> MGRDPNSTNDTTTQNVVLTKYGFDKDVTAIDRATDQIWTGDGAKPLQGVDFTIYNVTANYWASPKDYKGSFDSAPVAATGTTNDKGQLTQALPIQSKDASGKTRAAVYLFHETNPRAGYNTSADFWLTLPAKAAADGNVYVYPKNVQKTTY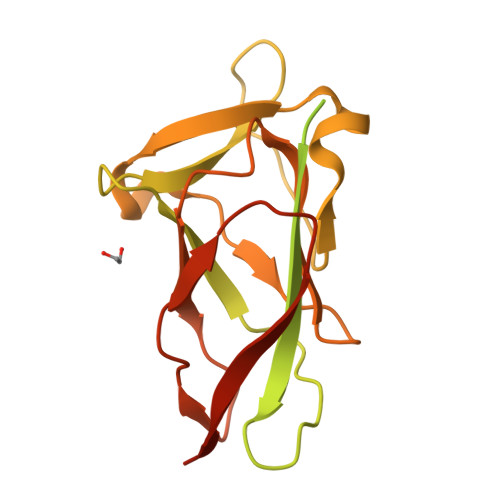ERTFVKKDAETKEVLEGAGFKISNSDGKFLKLTDKDGQSVSIGEGFIDVLANNYRLTWVAESDATVFTSDKSGKFGLNGFADNTTTYTAVETNVPDGYDAAANTDFKADNSSSDILDAPSGILPLEHHHHHH> AWPKVQPEVNIGVVGHVDHGKTTLVQAITGIWTSKHSEELKRGMTIKLGYAETNIGVCESCKKPEAYVTEPSCKSCGSDDEPKFLRRISFIDAPGHEVLMATMLSGAALMDGAILVVAANEPFPQPQTREHFVALGIIGVKNLIIVQNKVDVVSKEEALSQYRQIKQFTKGTWAENVPIIPVSALHKINIDSLIEGIEEYIKTPYRDLSQKPVMLVIRSFDVNKPGTQFNELKGGVIGGSIIQGLFKVDQEIKVLPGLRVEKQGKVSYEPIFTKISSIRFG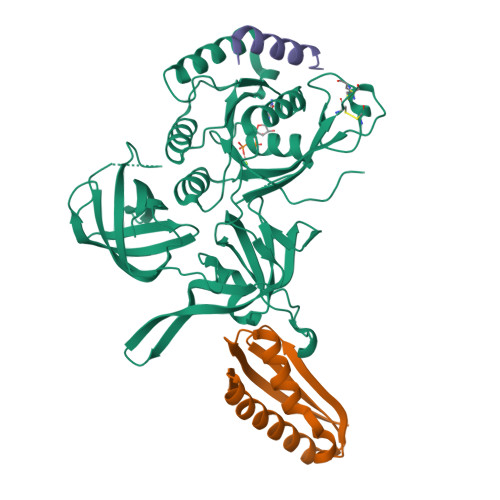DEEFKEAKPGGLVAIGTYLDPSLTKADNLLGSIITLADAEVPVLWNIRIKYNLLERVVGAKEMLKVDPIRAKETLMLSVGSSTTLGIVTSVKKDEIEVELRRPVAVWSNNIRTVISRQIAGRWRMIGWGLVEI;> MRKVKMSGLITVRTNEPLGVEKIKEVISKALENIEQDYESLLNIKIYTIGAPRYRVDVVGTNPKEASEALNQIISNLIKIGKEENVDISVVKK;> SSEKEYVEMLDRLYSKLP Mammalian target of rapamycin complex 1 (mTORC1) serves as a central regulator of cell growth and proliferation by integrating signals from growth factors, nutrients, energy status, and cellular stress. A small GTPase, called Ras homolog enriched in brain (Rheb), is a positive regulator of mTORC1. Like other small GTPases, the function of Rheb is dictated by its guanine nucleotide binding states: it is active in the GTP-bound form and inactive in the GDP-bound form. The Y35N mutant assumes a very similar overall structure as the WT Rheb with a typical small GTPase protein fold composed of a six-stranded β-sheet surrounded by four α-helices.

Surprisingly, the Y35N mutant, which was initially identified in several human cancers (Lawrence et al., 2014), could significantly increase the phosphorylation level of mTORC1 substrate S6K1 compared to the wild-type (WT) Rheb, and thus is regarded as a constitutively active mutant (Grabiner et al., 2014; Heard et al., 2014). To investigate the molecular basis for the constitutive activation of mTORC1 by the Y35N mutant, we determined the crystal structures of Y35NGppNHp and Y35NGDP at 2.0 Å and 2.1 Å resolution, respectively. The overall structure of Y35NGppNHp is very similar to that of WTGppNHp; superposition of the two structures using the secondary-structure matching method yields a root mean square deviation (RMSD) of 0.45 Å for 169 Cα atoms. In the Y35NGppNHp structure, there is a Mg2+ bound at the active site, which is coordinated by the side chains of Ser20 and Thr38, the β-phosphate and γ-phosphate of GppNHp, and two water molecules in an octahedral geometry. In WTGppNHp, the side chain of Tyr35 covers on the top of the phosphate-binding pocket and forms a hydrogen bond with the γ-phosphate of GppNHp. In Y35NGppNHp, the side chain of Asn35 flips into the bottom of the phosphate-binding pocket and points toward the α-phosphate and β-phosphate of GppNHp (about 90° rotation relative to that of Tyr35 in WTGppNHp). Besides, the binding modes of GppNHp and Mg2+ are essentially identical to those in WTGppNHp. In particular, Thr38 makes a coordination bond with Mg2+ via its side chain and forms hydrogen bonds with the γ-phosphate of GppNHp via its main chain and side chain. When the WT and Y35N Rheb structures are superimposed onto the Rheb‒mTORC1 structure, residues Pro37 and Ile39 of switch I in both WTGppNHp and Y35NGppNHp could interact with Phe977 and Arg1301 of mTOR. In other words, Y35NGDP mimics WTGppNHP in binding to mTOR and thus is capable to activate mTORC1 in a similar way as WTGppNHp. These results indicate that the Y35N mutation induces switch I in either GDP-bound or GppNHp-bound form to adopt a conformation similar to that seen in WTGTP and thus can make a tight interaction with mTOR, leading to constitutive activation of mTORC1.

> MPQSKSRKIAILGYRSVGKSSLTIQFVEGQFVDSNDPTIENTFTKLITVNGQEYHLQLVDTAGQDEYSIFPQTYSIDINGYILVYSVTSIKSFEVIKVIHGKLLDMVGKVQIPIMLVGNKKDLHMERVISYEEGKALAESWNAAFLESSAKENQTAVDVFRRIILEAEKLEHHHHHH>MVAPLLKTLPFLAAAYAAELDLPNFSALNRRQDNSTSSSAGCSLDQTVAPGNLTLCGNATLFTTFRPKARFIAPEGWMNAPMGLYQRADGSIHAGYQSHPKHIQWGNISQGAAYSSDFTSWTDFNGSEGYKTIWPSQIYDIRGVFDGSIIKEGIDGYPTILYTSTSFGPLGATLNEAEGTETQSLAYTTDDGASWIKLGYGAGQNPVIYEWPETNLTGFRDPYVFQSPRLEALLANTTSITNATGDHFATISGGVHGDGARLFLYRQHTTGEFIKWTYLGPLVTTGYKESYGEWSGNYGINFETAGVTRLNPAGAAWDNGSDTTAVDFVTFGTEQGRADHQNHWPLWAAVDYEVRDNGSIEAVIAYSGVQDWGRSYAYASFPVEGYRQVSVGWIYEDDDNVILAKQFGYQGAFTLFRDLFVKVVENVSPSTPGLFEQASWSTKNSTDGMSVTVTTLGQR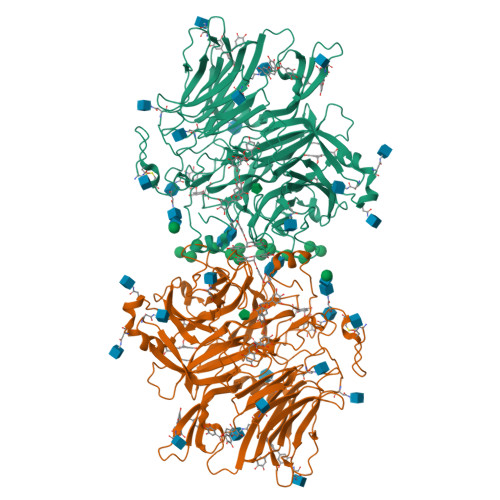VVPETLAAYKGNSTVSTLAPVMLNESAAAYTPFSSQPTDRFYALTGSFEFGLNTTAKAGFRVLASEEEYTDIWFDPASENLTVVRTASSLIKSFGNDTELAKVKLYEIVGAESKTLNLTVFVDGSVIEIYANDEVALSTRAYPWLANSTGAGLLADGTTAGDVVGVSGLELWDGLVDAWPARPANTSQGLVWDGPTAAMYGLFAGY[2x]> QIRYSVPEETDKGTVVGNISKDLGLEPRELAERGVRIVSRGRSQLFSLNPRGGSLVTAGRIDREELCAQSTPCLVNINILVEEKGKLFGVEIEITDINDNNPKFHVGDLEVKINEIAAPGARYPLPEAVDPDVGINSLQSYQLSPNRHFSLHLQTGDDGTINPELVLERTLDREEEPTHHLVLTASDGGEPRRSSTALIQITVLDTNDNAPVFDQPVYRVKVLENVAPGTLLLTVRASDPDEGVNGKVTYKFRKINEKQSLLFHLHENTGEMTVAKNLDYEECSLYEMEIQAEDVGALLGRSKVIIMVEDVNDNRPEVTITSLFNPVLENSLPGTVIAFLNVHDQDSGKNGQVVCYTHDNLPFKLEKSIDNYYRLVTWKYLDREKVSTYNITVIASDLGAPPLSTETYIALTVADTNDHHHHHHHH

By contrast, in vertebrates the clustered protocadherins (Pcdhs) provide analogous cell-surface diversity, but in this case generated through stochastic alternative promoter choice. Biophysical measurements with domain-deleted proteins showed that Pcdhs also interact in cis, through a membrane-proximal dimer interface involving extracellular cadherin domain 6 (EC6) and potentially EC5. The specificity-determining cell-cell recognition interface of Pcdhs involves domains EC1–4, as shown experimentally through mutagenesis analysis and suggested by mutation correlation analysis.

The γA8EC1–4 crystal structure contained a single molecule in the asymmetric unit, which is engaged with a symmetry mate in an anti-parallel EC2–3-mediated interaction involving the same surface of the molecule as in the other clustered Pcdh trans dimer structures. This crystal also contained a distinct interaction between symmetry-related molecules, also mediated by an anti-parallel EC2–3 interface and with a similar buried surface area. In order to confirm which interface is the biological trans dimerization interface, we generated a number of γA8 arginine mutants separately targeting each of the observed interactions. Only those mutants that targeted the interaction surface in common with other Pcdhs resulted in loss of function in cell aggregation assays. It is this γA8 dimer interaction that is shown in Figure 1A. Remarkably, like the γA1EC1–4 dimer observed between chains C and D, the EC1:EC4 interaction is not formed. However, in the case of γA8 the interaction surfaces of EC1 and EC4 instead make contacts with the EC4 domain of another symmetry-related molecule in the crystal. Since we have not observed molecular species larger than a dimer for Pcdh EC1–4 fragments we believe this alternative EC1:EC4 interaction, as well as the additional EC2:EC3 interaction, to be an artifact of crystallization. The absence of this interaction in some of the γA crystal structures is therefore likely an artifact of crystallization, perhaps due to crystallization condition, although it does imply that the EC1:EC4 interaction is not particularly stable.>EEGLDFPEYDGVDRVVNVNAKNYKNVFKKYEVLALLYHEPPEDDKASQRQFEMDELILELAAQVLEDKGVGFGMVDSEKDAAVAKKLGLTEEDSVYVFKGDEVIEYDGEFSADTLVEFLLDVLEDPVELIEGERELQAFENIEDDNKLIGYFKNKDSEHYKAYEDAAEEFHPYIPFFATFDSKVAKKLTLKLNEIDFYEAFMEEPVTIPDKPNSEEEIVSFVEAHKRSTLRKLKPESMYETWEDDLDGIHIVAFAEETDPDGYEFLETLKAVAQDNTDNPDLSIIWIDPDDFPLLVPYWEKTFNIDLSAPQIGVVNVTDADSVWMEMDDEEDLPSAEELEDWLEDVLEGEINTEDDDEEDD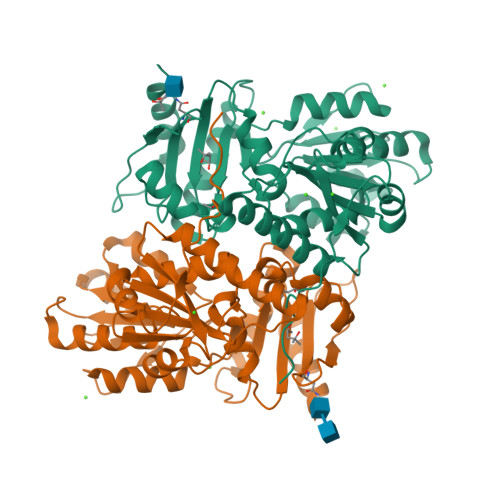[4x]> GAMGSMGTRDDEYDYLFKVVLIGDSGVGKSNLLSRFTRNEFNLESKST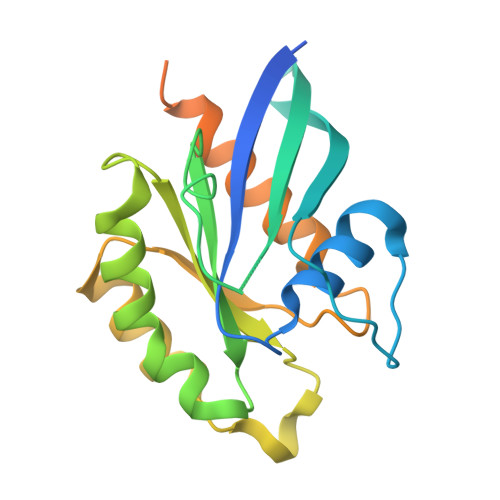IGVEFATRSIQVDGKTIKAQIWDTAGQERYRAITSAYYRGAVGALLVYDIAKHLTYENVERWLKELRDHADSNIVIMLVGNKSDLRHLRAVPTDEARAFAEKNGLSFIETSALDSTNVEAAFQTILTEIYRIVSQKQMSDRRENDMSPSNNVVPIHVPPTTENKPKVQCCQNI> MSQEALKAPVVVLGAGLASVSFVAELRQAGYQGLITVVGDEAERPYDRPPLSKDFMAHGDAEKIRLDCKRAPEVEWLLGVTAQSFDPQAHTVALSDGRTLPYGTLVLATGAAPRALPTLQGATMPVHTLRTLEDARRIQAGLRPQSRLLIVGGGVIGLELAATARTAGVHVSLVQRGPRLMSRAAPATLADFVARYHAAQGVDLRFERSVTGSVDGVVLLDDGTRIAADMVVVGIGVLANDALARA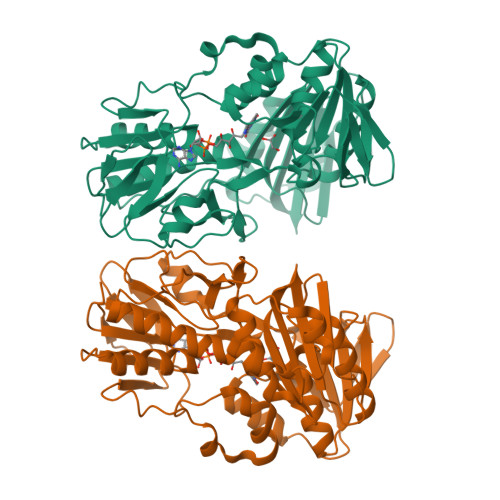AGLACDDGIFVDAYGRTTCPDVYALGDVTRQRNPLSGRFERIETWSNAQNQGIAVARHLVDPTAPGYAELPWYWSDQGALRIQVAGLASGDEEIVRGEVSLDAPKFTLIELQKGRIVGATCVNNARDFAPLRRLLAVGAKPDRAALADPATDLRKLAAAVAA> KDVPPKQLRFEGERVTWIQASTLKELLDLKAQHPEAKLVVGNTEIGIEMKFKNQLFPMIICPAWIPELNAVEHGPEGISFGAACALSSVEKTLLEAVAKLPTQKTEVFRGVLEQLRWFAGKQVKSVASLGGNIITASPISDLNPVFMASGTKLTIVSRGTRRTVPMDHTFFPSYRKTLLGPEEILLSIEIPYSREDEFFSA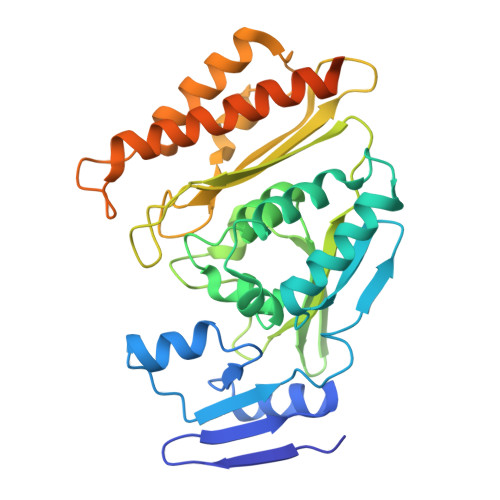FKQASRREDDIAKVTCGMRVLFQPGSMQVKELALCYGGMADRTISALKTTQKQLSKFWNEKLLQDVCAGLAEELSLSPDAPGGMIEFRRTLTLSFFFKFYLTVLKKLGKDSKDKCGKLDPTYTSATLLFQKHPPANIQLFQEVPNGQSK>GQSAKEAIEAALADFVKAYNSKDAAGVASKYMDDAAIFPLDMARVDGRQNIQKLWQGLMDMGVSEPKLTTLDVQESGDFAFESGSISLKGPGKDSKLVDIAGKYVEVWRKGQDGGWKLYRTIANLDPAKLEHHHHH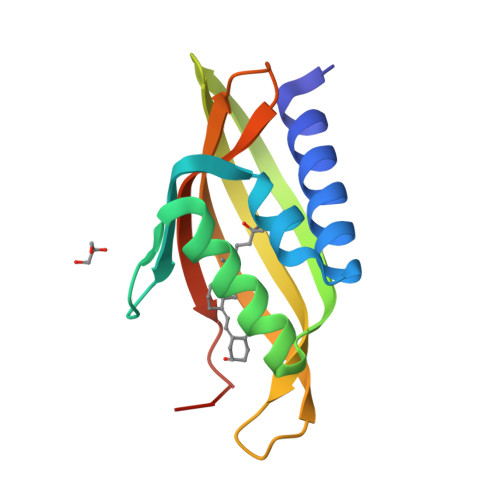H[2x]> ACDYTCGSNCYSSSDVSTAQAAGYQLHEDGETVGSNSYPHKYNNYE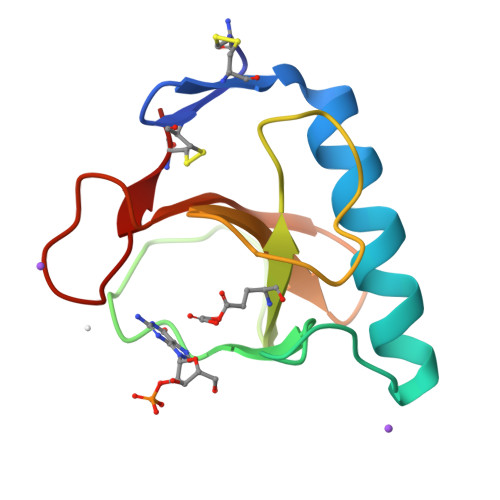GFDFSVSSPYYEWPILSSGDVYSGGSPGADRVVFNENNQLAGVITHTGASGNNFVECT> MEEIEHRTVEVNGIKMHVAEKGEGPVVLFLHGFPELWYSWRHQILALSSRGYRAVAPDLRGYGDTEAPVSISSYTGFHIVGDLIALIDLLGVDQVFLVAHDWGAIIGWYLCTFHPDRVKAYVCLSVPLLHRDPNIRTVDAMRAMYGDDYYICRFQKPGEMEAQMAEVGTEYVLKNILTTRKPGPPIFPKGEYGTGFNPDMPNSLPSWLTQDDLAYYVSKYEKTGFTGPLNYYRNMNLNWELTAPWSGGKIQVPVKFITGELDNVYTSLNMKEYIHGGGFKQDVPNLEEVIVQKNVAHFNNQEAAEEINNHIYDFIKKF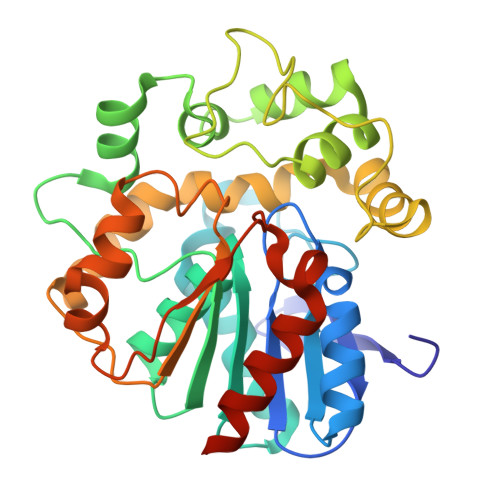LEHHHHHH> MYYALLTLFVIIAVVLIISTLLQKGRGDVGAAFGGGMGQSIFGVGGVETILTKATYWLGALFLVLALLLSVIPKEKGSVVEKSVQTEQSE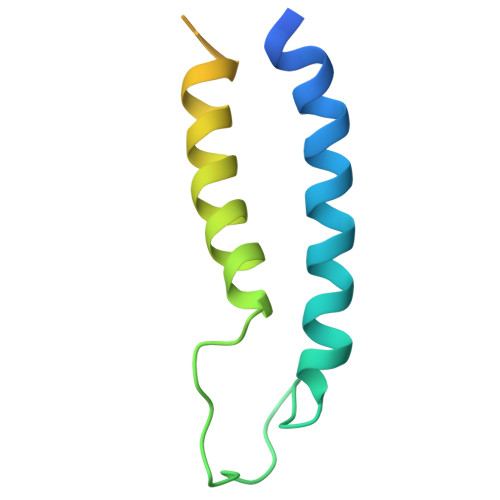GKGTTQESGKGHHHHHH> MGSSHHHHHHSSGENLYFQGHMLRISQEALTFDDVLLIPGYSEVLPKDVSLKTRLTRGIELNIPLVSAAMDTVTEARLAIAMAQEGGIGIIHKNMGIEQQAAEVRKVKKHETAIVRDPVTVTPSTKIIELLQMAREYGFSGFPVVEQGELVGIVTGRDLRVKPNAGDTVAAIMTPKDKLVTAREGTPLEEMKAKLYENRIEKMLVVDENFYLRGLVTFRDIEKAKTYPLASKDEQGRLRVGAAVGTGADTGERVAALVAAGVDVVVVDTAHGHSKGVI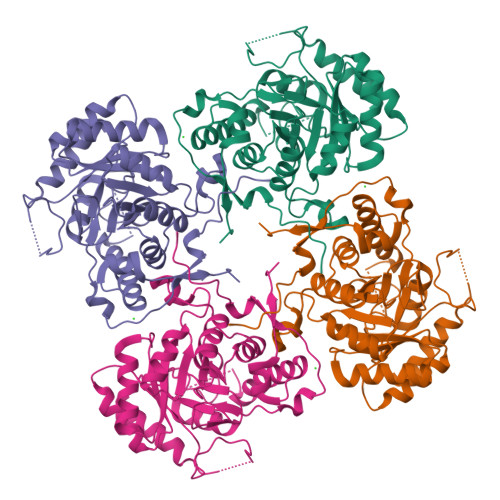ERVRWVKQTFPDVQVIGGNIATAEAAKALAEAGADAVKVGIGPGSICTTRIVAGVGVPQISAIANVAAALEGTGVPLIADGGIRFSGDLAKAMVAGAYCVMMGSMFAGTEEAPGEIELFQGRSYKSYRGMGSLGAMSGSQGSSDRYFQDASAGAEKLVPEGIEGRVPYKGALSAIVHQLMGGLRAAMGYTGSADIQQMRTQPQFVRITGAGMAESHVHDVQITKEAPNYRVG>[4x]MKQGFEFNIMVVGQSGLGKSTLINTLFKSKISRKSVQPTSEERIPKTIEIKSITHDIEEKGVRMKLTVIDTPGFGDHINNENCWQPIMKFINDQYEKYLQEEVNINRKKRIPDTRVHCCLYFIPATGHSLRPLDIEFMKRLSKVVNIVPVIAKAD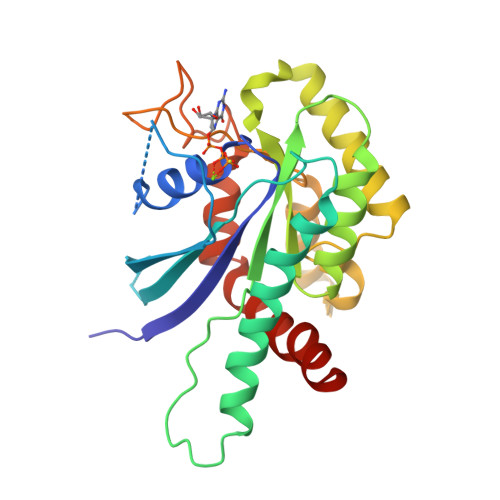TLTLEERVHFKQRITADLLSNGIDVYPQKEFDEDSEDRLVNEKFREMIPFAVVGSDHEYQVNGKRILGRKTKWGTIEVENTTHCEFAYLRDLLIRTHMQNIKDITSSIHFEAYRVKRLN>[4x]GDELYRQSLEIISRYLREQATGAKDTKPMGRSGATSRKALETLRRVGDGVQRNHETAFQGMLRKLDIKNEDDVKSLSRVMIHVFSDGVTNWGRIVTLIS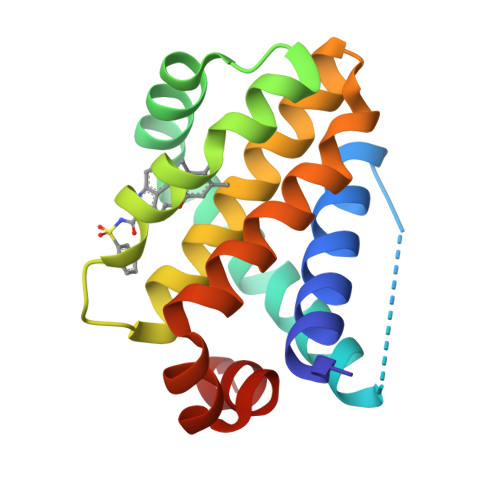FGAFVAKHLKTINQESCIEPLAESITDVLVRTKRDWLVKQRGWDGFVEFFH> KKIFKPEELRQALMPTLEALYRQDPESLPFRQPVDPQLLGIPDYFDIVKNPMDLSTIKRKLDTGQYQEPWQYVDDVWLMFNNAWLYNR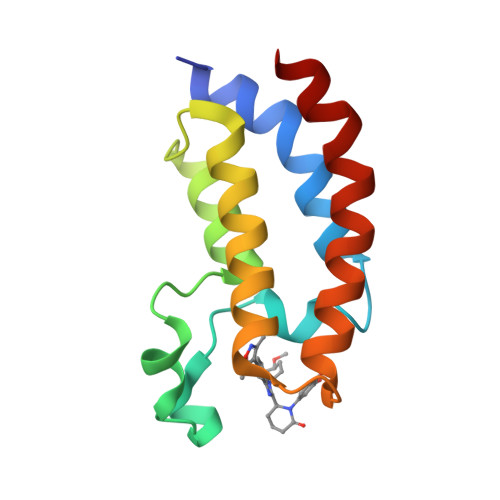KTSRVYKFCSKLAEVFEQEIDPVMQSLG> MNAHLANEVQYDLGHPSSLVHVIISSECLAAAGIPLAALMRANFQVEIQTRAHATGDCTPWCTAFAAYVPADAVGELLAPVVPAHPGLLPRASSAGGLFVSLPVVCDAQGVYDPYAVAALRLAWGSGASCARVILFSYDELVPPNTRYAADSTRIMRVCRHLCRYVALLGAAAPPAAKEAAAHLSMGLPPISPEEQLTAPGGDTTAAQDVSIAQENEEILALVQRRSLVEWLDRGWEALAGGD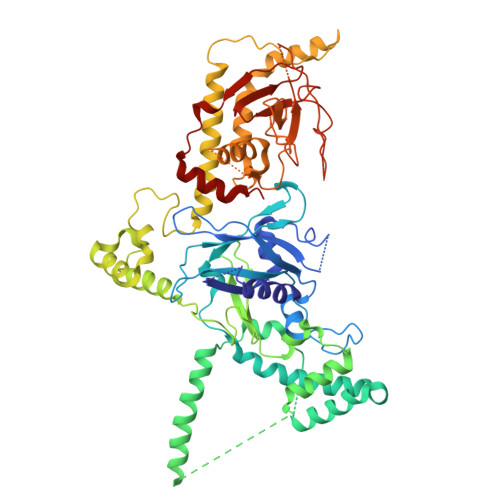RPDWLWSRRSISVVLRHHYGTKQRFVVVSYENSVAWGGRRARPPLLSSALATALTEACAAERVVRPHQLSPAGQAELLLRFPALEVPLRHPRPVLPPFDIAAEVAFTARIHLACLRALGQAIRAALQGGPRISQRLRYDFGPDQRAWLGEVTRRFPILLENLMRAVEGTAPDAFFHTAYALAVLAHLGGRVVPLGDDLPARFADSDGHYVFDYYSTSGDTLRLNNRPIAVAMDEQSKCRFMEAPRRVCEQYLPGESYAYLCLGFNRRLCGIVVFPGGFAFTINIAAYLSLSDPVARAAVLRFCRKVS>GSHMASMKPIFDINETFEKQLKDLTSNVKSIQDNLLEEIITPNTKTEYLQRFLIDRFDKELFKKNVP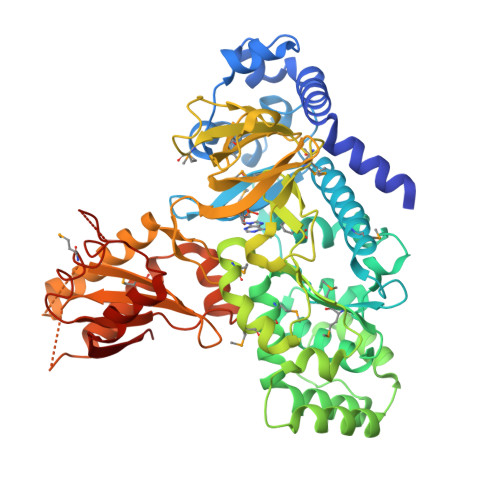IVSYEDIKPYLDRVVNGESSDVISARTITGFLLSSGTSGGAQKMMPWNNKYLDNLTFIYDLRMQVITKHVKGVEEGKGMMFLFTKQESMTPSGLPARVATSSYFKSDYFKNRPSNWYYSYTSPDEVILCPNNTESLYCHLLCGLVQRDEVVRTGSIFASVMVRAIEVLKNSWEELCSNIRSGHLSNWVTDLGCQNSVSLVLGGPRPELADTIEEICNQNSWKGIVKRLWPNTKYIETVVTGSMGQYVPMLNYYCNDLPLVSTTYGSSETTFGINLDPLCKPEDVSYTFMPNMSYFEFIPMDGGDKNDVVDLEDVKLGCTYEPVVTNFAGLYRMRVGDIVLVTGFYNNAPQFKFVRRENVVLSIDSDKTNEEDLFKAVSQAKLVLESSGLDLKDFTSYADTSTFPGHYVVYLEVDTKEGEEKETAQFELDEEALSTCCLVMEESLDNVYKRCRFKDGSIGPLEIRVVRQGTFDSLMDFFISQGASTGQYKTPRCIKSGKALQVLETCVVAKFFSI[2x]> MGTRDDEYDYLFKVVLIGDSGVGKSNLLSRFTRNEFNLESKSTIGVEFATRSIQVDGKTIKAQIWDTAGQERYRAITSAYYRGAVGALLVYDIAKHLTYENVERWLKELRDHADSNIVIMLVGNKSDLRHLRAVPTDEARAFAEKNGLSFIETSALDSTNVEAA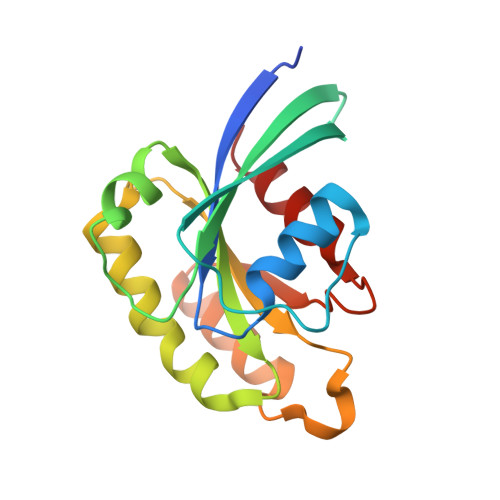FQTILTEIY>[3x]EMVKKITSMNRGDFKQITLATGAGKTTELPKAVIEEIGRHKRVLVLIPLRAAAESVYQYMRLKHPSISFNLRIGDMKEGDMATGITYASYGYFCQMPQPKLRAAMVEYSYIFLDEYHCATPEQLAIIG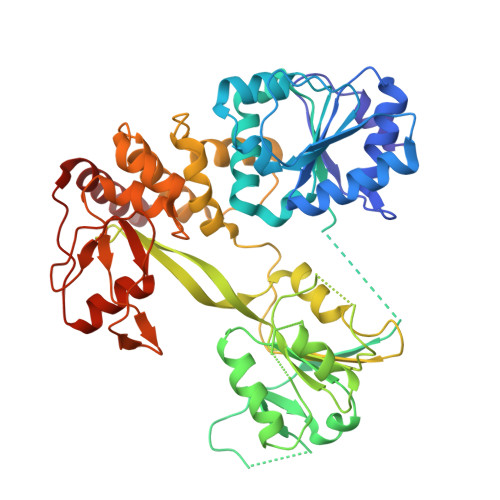KIHRFSESIRVVAMTATPAGSVTTTGQKHPIEEFIAPEVMKGEDLGSQFLDIAGLKIPVDEMKGNMLVFVPTRNMAVEVAKKLKAKGYNSGYYYSGEDPANLRVVTSQSPYVIVATNAIESGVTLPDLDTVIDTGLKCEKRVRVSSKIPFIVTGLKRMAVTVGEQAQRRGRVGRVKPGRYYRSQETATGSKDYHYDLLQAQRYGIEDGINVTKSFREMNYDWSLYEEDSLLITQLEILNNLLISEDLPAAVKNIMARTDHPEPIQLAYNSYEVQVPVLFPKIRNGEVTDTYENYSFLNARKLGEDVPVYIYATEDEDLAVDLLGLDWPDPGNQQVVETGKALKQVTGL Type 4 pili (T4P)—important in bacterial pathogens—are filaments composed of one well-characterized major pilin, and several minor pilins whose roles are often poorly understood. Streptococcus sanguinis T4P are composed of five pilins, which makes it a good model to determine the role of each pilin subunit in detail. PilE1/PilE2 are the major pilins forming the backbone of the filament, while the three minor pilins (PilA, PilB, and PilC) form a tip-located complex promoting adhesion to various host receptors. Here, we characterize PilA and PilC, showing how they interact and how they function.

Protein crystals for PilCSK36 were produced in 0.2 µL sitting drop with a 1:1 protein to mother liquor (0.2 M MgCl26H2O, 20% w/v PEG 3350). Data were collected at the Diamond beamline i04, and structure was produced using the PilC structure from strain 2908 for molecular replacement. After collecting a complete dataset, we solved a 1.60 Å resolution structure. Surprisingly, although the purified protein contained the pilin moiety, this portion was missing in the crystals. It must therefore have been degraded during prolonged incubation in the crystallization trays due to its inherent instability. When we compared our two PilC structures, we found that they are essentially identical, superposing onto each other with an rmsd of only 0.79 Å. This suggests that these proteins—showing 57% sequence identity —are likely to bind similar glycan ligands. We observed a similar binding profile for PilCSK36, showing that glycan-binding ability is conserved in PilC orthologs.

> STGYQNILGQRNQNALNFDIQEDFETRLAKIKKDGGSGNDVEIFTYRIGKNGRSNSVSVKGTTLSYKDNKVKNIHLFAANKKEIPLDIPEDLVVSLKDTNRYYYYAGETGPAGQAGFKDNKQSTKAKIHTSSAWFLSESSINYNNSRIVPVGTLGSNVQDQGFGIVLPKLPDDFQQISSNEKPIAITDEMRGRYLTFAARGINSFGRVGKYQEGPQRIWVMGLPNRGMRSNLVLHTDADLALMRNSDNTISAIPADGVAHTNTVVANYAETKKNGVYGAVIPVINYKEPAINQTRQLIALNDSKIQFSNHDFNKGYTTSMLIGNRQQTGSLLTYKLDNSLNWTVSLEANGKIAIETVDNTNANNGGRQYANVVLDYTKDNSIQVRASVTNKILTLEVFVNGALVHTHELFMERNGVTHDIRKSQIIFGGKTFINEFAVYNKKLTDSEINILAEYFSDKYRAKA Here we used *de novo* model building to identify a protein contaminant within a recombinantly-expressed protein sample as the helical tail of the YDC107 bacteriophage. All top 100 hits pointed to the *Escherichia coli* phage tail protein, specifically phage YDC107 – an unclassified *Ravinvirus* from a *Caudioviricetes* class. Structural analysis revealed that the central part of the phage tail has a C6 symmetry, however the overall symmetry of each segment is C3 due to dimerization of a flexible domain.

After two rounds of 2D classification, where only classes with sharp details were selected ([Fig figS2]), a total of 5,927 particles were used for *ab-initio* map generation and refinement ([Fig fig1], [Fig figS2]). The final map had a reported GSFSC resolution of 3.22 Å and was b-factor corrected based on the estimation from a Guinier plot ([Fig figS3]). This final map was used for structure prediction and model building of the phage tail’s core. We chose the top max score sequence with accession code MCN3709170.1 as our reference sequence. Comparison between the DeepTracer model and AlphaFold models revealed that only residues 1-154 were predicted by DeepTracer ([Fig fig3]). This corresponds to visual inspection of the C6-helical refined map in Coot – there were no unmodelled densities. However, the AlphaFold model suggested the presence of an additional β-sheet domain connected to the central core by a flexible linker ([Fig fig3], magenta). Low-pass filtering the C6-helical map to 12 Å resolution revealed the presence of extra protruding domains that could potentially accommodate the unmodelled flexible domain that was observed in the AlphaFold prediction ([Fig fig4]). We used AlphaFold multimer to generate five models of the flexible domain dimer ([Fig fig4]), all of which formed a C2-symmetric arrangement and fit well into the observed unmodelled density. Due to the flexible domain dimerization, individual phage tail monomers can exist in two conformations: forward and reverse ([Fig fig5]).

>[6x]MPTPNPLPVKGAGTTLWVYKGNGDPYANPLSDVDWSRLAKVKDLTPGELTAESYDDSYLDDEDADWTATGQGQKSAGDTSFTLAWMPGEQGQQALLAWFNEGDTRAYKIRFPNGTVDVFRGWVSSIGKAVTAKEVITRTVKVTNVGRPSMAEDRSTVTAATGMTVTPASASVVKGQSTTLTVAFQPEGATDKSFRAVSSDKTKATVSVSGMTITVNGVAAGKVNIPVVSGNGEFAAVAEITVTAS> MDSLSVNQILYPEVHLDSPIVTNKIVAILEYARVPHAYSLEDPTLCQNIKHRLKNGFSNQMIINNVEVGNVIKSKLRSYPAHSHIPYPNCNQDLFNIEDKESTRKIRELLKKGNSLYSKVSDKVFQCLRDTNSRLGLGSELREDIKEKVINLGVYMHSSQWFEPFLFWFTVKTEMRSVIKSQTHTCHRRRHTPVFFTGSSVELLISRDLVAIISKESQHVYYLTFELVLMYCDVIEGRLMTETAMTIDARYTELLGRVRYMWKLIDGFFPALGNPTYQIVAMLEPLSLAYLQLRDITVELRGAFLNHCFTEIHDVLDQNGFSDEGTYHELIEALDYIFITDDIHLTGEIFSFFRSFGHPRLEAVTAAENVRKYMNQPKVIVYETLMKGHAIFCGIIINGYRDRHGGSWPPLTLPLHAADTIRNAQASGDGLTHEQCVDNWKSFAGVKFGCFMPLSLDSDLTMYLKDKALAALQREWDSVYPKEFLRYDPPKGTGSRRLVDVFLNDSSFDPYDVIMYVVSGAYLHDPEFNLSYSLKEKEIKETGRLFAKMTYKMRACQVIAENLISNGIGKYFKDNGMAKDEHDLTKALHTLAVSGVPKDLKESHRGGPVLKTYSRSPVHTSTRNVRAAKGFIGFPQVIRQDQDTDHPENMEAYETVSAFITTDLKKYCLNWRYETISLFAQRLNEIYGLPSFFQWLHKRLETSVLYVSDPHCPPDLDAHIPLYKVPNDQIFIKYPMGGIEGYCQKLWTISTIPYLYLAAYESGVRIASLVQGDNQTIAVTKRVPSTWPYNLKKREAARVTRDYFVILRQRLHDIGHHLKANETIVSSHFFVYSKGIYYDGLLVSQ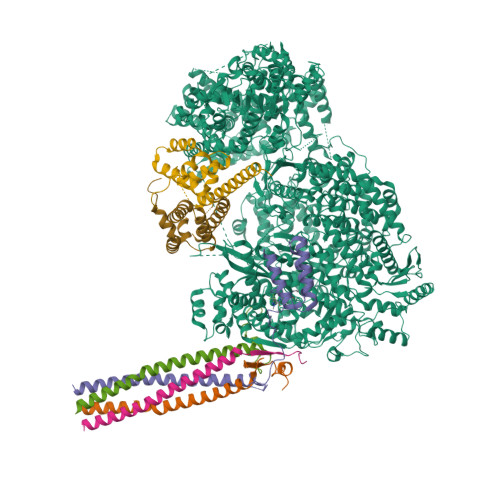SLKSIARCVFWSETIVDETRAACSNIATTMAKSIERGYDRYLAYSLNVLKVIQQILISLGFTINSTMTRDVVIPLLTNNDLLIRMALLPAPIGGMNYLNMSRLFVRNIGDPVTSSIADLKRMILASLMPEETLHQVMTQQPGDSSFLDWASDPYSANLVCVQSITRLLKNITARFVLIHSPNPMLKGLFHDDSKEEDEGLAAFLMDRHIIVPRAAHEILDHSVTGARESIAGMLDTTKGLIRASMRKGGLTSRVITRLSNYDYEQFRAGMVLLTGRKRNVLIDKESCSVQLARALRSHMWARLARGRPIYGLEVPDVLESMRGHLIRRHETCVICECGSVNYGWFFVPSGCQLDDIDKETSSLRVPYIGSTTDERTDMKLAFVRAPSRSLRSAVRIATVYSWAYGDDDSSWNEAWLLARQRANVSLEELRVITPISTSTNLAHRLRDRSTQVKYSGTSLVRVARYTTISNDNLSFVISDKKVDTNFIYQQGMLLGLGVLETLFRLEKDTGSSNTVLHLHVETDCCVIPMIDHPRIPSSRKLELRAELCTNPLIYDNAPLIDRDATRLYTQSHRRHLVEFVTWSTPQLYHILAKSTALSMIDLVTKFEKDHMNEISALIGDDDINSFITEFLLIEPRLFTIYLGQCAAINWAFDVHYHRPSGKYQMGELLSSFLSRMSKGVFKVLVNALSHPKIYKKFWHCGIIEPIHGPSLDAQNLHTTVCNMVYTCYMTYLDLLLNEELEEFTFLLCESDEDVVPDRFDNIQAKHLCVLADLYCQPGTCPPIQGLRPVEKCAVLTDHIKAEAMLSPAGSSWNINPIIVDHYSCSLTYLRRGSIKQIRLRVDPGFIFDALAEVNVSQPKIGSNNISNMSIKAFRPPHDDVAKLLKDINTSKHNLPISGGNLANYEIHAFRRIGLNSSACYKAVEISTLIRRCLEPGEDGLFLGEGSGSMLITYKEILKLSKCFYNSGVSANSRSGQRELAPYPSEVGLVEHRMGVGNIVKVLFNGRPEVTWVGSVDCFNFIVSNIPTSSVGFIHSDIETLPDKDTIEKLEELAAILSMALLLGKIGSILVIKLMPFSGDFVQGFISYVGSHYREVNLVYPRYSNFISTESYLVMTDLKANRLMNPEKIKQQIIESSVRTSPGLIGHILSIKQLSCIQAIVGDAVSRGDINPTLKKLTPIEQVLINCGLAINGPKLCKELIHHDVASGQDGLLNSILILYRELARFKDNQRSQQGMFHAYPVLVSSRQRELISRITRKFWGHILLYSGNRKLINKFIQNLKSGYLILDLHQNIFVKNLSKSEKQIIMTGGLKREWVFKVTVKETKEWYKLVGYSALIKD;>[4x]MAEEQARHVKNGLECIRALKAEPIGSLAIEEAMAAWSEISDNPGQERATCREEKAGSSGLSKPCLSAIGSTEGGAPRIRGQGPGESDDDAETLGIPPRNLQASSTGLQCHYVYDHSGEAVKGIQDADSIMVQSGLDGDSTLSGGDNESENSDVDIGEPDTEGYAITDRGSAPISMGFRASDVETAEGGEIHELLRLQSRGNNFPKLGKTLNVPPPPDPGRASTSGTPIKKGTDARLASFGTEIASSLTGGATQCARKSPSEPSGPGAPAGNVPECVSNAALIQEWTPESGTTISPRSQNNEEGGDHYDDELFSDVQDIKTALAKIHEDNQKIISKLESLLLLKGEVESIKKQINRQNISISTLEGHLSSIMIAIPGLGKDPNDPTADVEINPDLKPIIGRDSGRALAEVLKKPVASRQLQGMTNGRTSSRGQLLKEFQLKPIGKKMSSAVGFVPDTGPASRSVIRSIIKSSRLEEDRKRYLMTLLDDIKGANDLAKFHQMLMKIIMKSG;>[2x]MSKTDWNASGLSRPSPSAHWPSRKLWQHGQKYQTTQDRSEPPAGKRRQAVRVSANHASQQLDQLKAVHLASAVRDLERAMTTLKLWESPQEISRHQALGYSVIMFMITAVKRLRESKMLTLSWFNQALMVIAPSQEETMNLKTAMWILANLIPRDMLSLTGDLLPSLWGSGLLMLKLQKEGRSTSS> MTPPLATTIDRLRDYLDRVGFQQ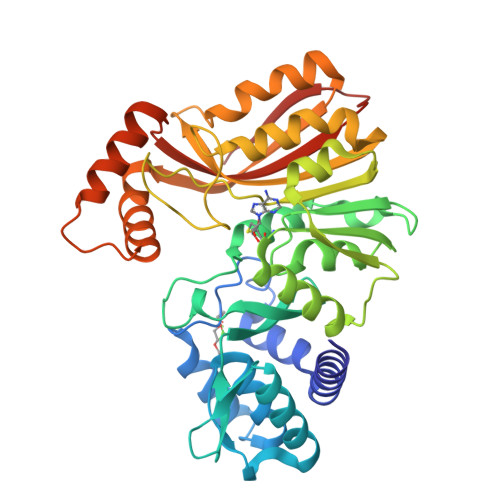IYKYIVAVNHYAVTPALITRNTAASVHHFFDSRLGGRAEFALLQCLMTGRPAEHAALPDKDRALADALVTAGLLRASPDGREVSGADRQLISAFGVDLLIDRRIHFGGEVHEVYIGPDSYWMLYYINASGIARTHRAVDLCTGSGIAALYLSLFTDHVLATDIGDVPLALVEINRRLNRRDAGTMEIRRENLNDTLDGRERFDLLTCAPPFVAFPPGYSGTLYSQGTGVDGLGYMRDIVGRLPEVLNPGGSAYLVADLCGDAHGPHFLGELESMVTGHGMRIEAFIDHVLPASAQVGPISDFLRHAAGLPADTDIAADVQAFQRETLRADYYYLTTIRLQTAAQNPGLRMLRRDPLPGAGT> MIVLFVDFDYFYAQVEEVLNPSLKGKPVVVCVFSGRFEDSGAVATANYEARKFGVKAGIPIVEAKKILPNAVYLPMRKEVYQQVSSRIMNLLREYSEKIEIASIDEAYLDISDKVRDYREAYNLGLEIKNKILEKEKITVTVGISKNKVFAKIAAD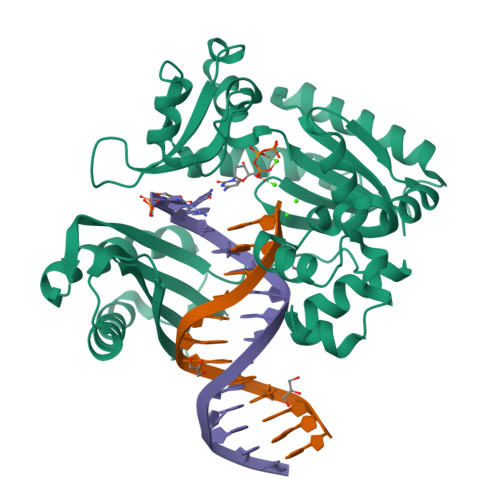MAKPNGIKVIDDEEVKRLIRELDIADVPGIGNITAEKLKKLGINKLVDTLSIEFDKLKGMIGEAKAKYLISLARDEYNEPIRTRVRKSIGRIVTMKRNSRNLEEIKPYLFRAIEESYYKLDKRIPKAIHVVAVTEDLDIVSRGRTFPHGISKETAYSESVKLLQKILEEDERKIRRIGVRFSKFIEAIGLDKFFDT>MHNDKDLSTWQTFRRLWPTIAPFKAGLIVAGVALILNAASDTFMLSLLKPLLDDGFGKTDRSVLVWMPLVVIGLMILRGITSYVSSYCISWVSGKVVMTMRRRLFGHMMGMPVSFFDKQSTGTLLSRITYDSEQVASSSSGALITVVREGASIIGLFIMMFYYSWQLSIILIVLAPIVSIAIRVVSKRFRNISKNMQNTMGQVTTSAEQMLKGHKEVLIFGGQEVETKRFDKVSNRMRLQGMKMVSASSISDPIIQLIASLALAFVLYAASFPSVMDSLTAGTITVVFSSMIALMRPLKSLTNVNAQFQRGMAACQTLFTILDSEQEKDEGK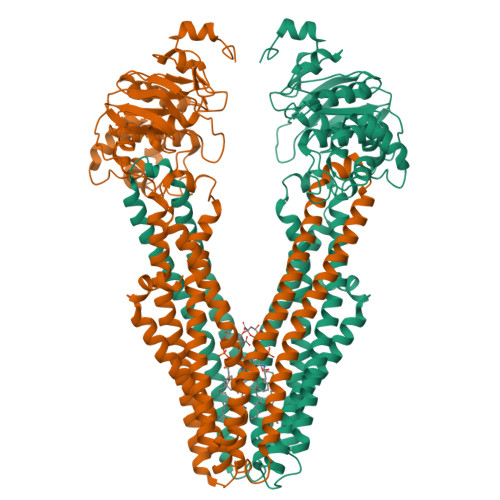RVIERATGDVEFRNVTFTYPGRDVPALRNINLKIPAGKTVALVGRSGSGKSTIASLITRFYDIDEGEILMDGHDLREYTLASLRNQVALVSQNVHLFNDTVANNIAYARTEQYSREQIEEAARMAYAMDFINKMDNGLDTVIGENGVLLSGGQRQRIAIARALLRDSPILILDEATSALDTESERAIQAALDELQKNRTSLVIAHRLSTIEKADEIVVVEDGVIVERGTHNDLLEHRGVYAQLHKMQFGQ[2x]(2~{R})-2-azanyl-~{N}-(4-ethanoyl-5-pyridin-3-yl-1,3-thiazol-2-yl)propanamide 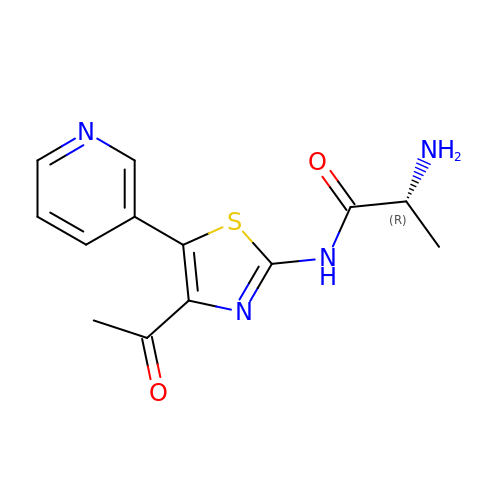| C13 H14 N4 O2 S | KLVIQLBTZDKJSI-SSDOTTSWSA-N> TSSANEDMPVERILEAELAVEPKTETYVEANMGLNPSSPNDPVTNICQAADKQLFTLVEWAKRIPHFSELPLDDQVILLRAGWNELLIASFSHRSIAVKDGILLATGLHVHRNSAHSAGVGAIFDRVLTELVSKMRDMQMDKTELGCLRAIVLFNPDSKGLSNPAEVEALREKVYASLEAYCKHKYPEQPGRFAKLLLRLPALRSIGLKCLEHLFFFKLIGD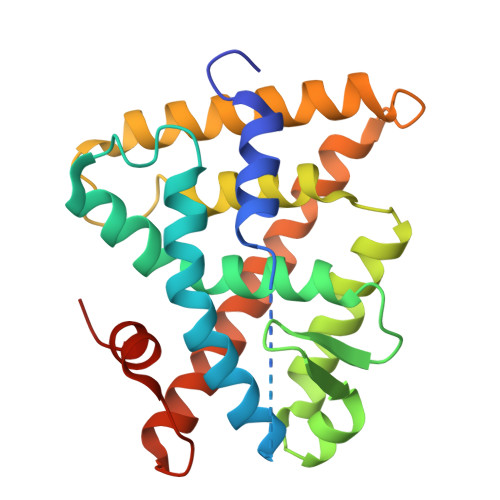TPIDTFLMEMLEAPHQMT>[2x]EYDYLFKVVLIGDSGVGKSNLLSRFTRNEFN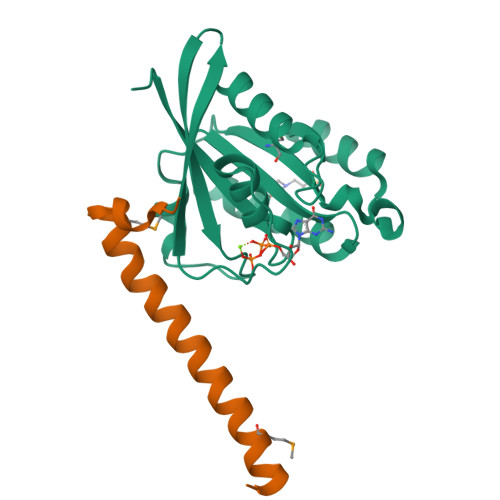LESKSTIGVEFATRSIQVDGKTIKAQIWDTAGLERYRAITSAYYRGAVGALLVYDIAKHLTYENVERWLKELRDHADSNIVIMLVGNKSDLRHLRAVPTDEARAFAEKNGLSFIETSALDSTNVEAAFQTILTEIY;>[2x]VSRDELMEAIQKQEEINFRLQDYIDRIIVAIMETNPSILEVK>[4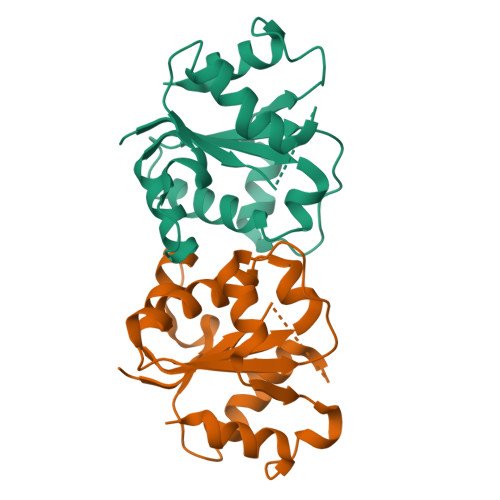x]MKDFDAFVSYAKWSSFPSEATSSLSEEHLALSLFPDVLENKYGYSLCLLERDVAPGGVYAEDIVSIIKRSRRGIFILSPNYVNGPSIFELQAAVNLALDDQTLKLILIKFCYFQEPESLPHLVKKALRVLPTVTWRGLKSVPPNSRFWAKMRYHMPVKLEHHHHHH> ATAILRPIGLHVEKFQQTYRKKWRFLTSANANVILAEAASGERPARWALTTGMASIPWEYLFFYMSPAEYNRMKNYPGTFAKSASVRIRTWNTRVAFQTGDTQTANATLNQNKFLQVAKGIRSIPFICSTNRKY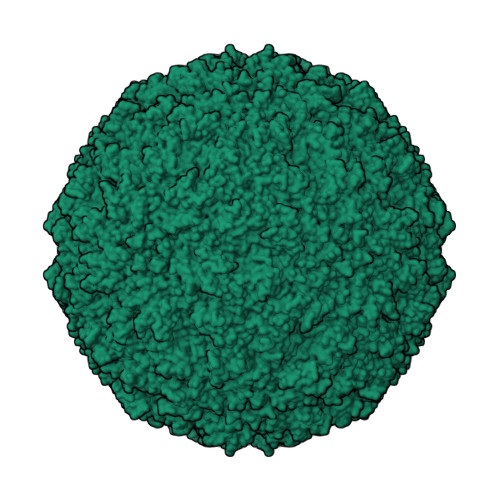TYSDTEPMQPTGFATLTSYEYRDGLKIAMYGYDNDSADFAKKPPADATGAEIYLQDYLTIYTNDARATTGTKILAGFPPYKNFIEEFDASACINTDVVAMDYDFSYAPLVPQFAPVPNNLITQNYNASYPAGTKNEVTAVKTTDSSQATPPTQVRNAPRKYIQGPNADTTFFDEEQNYLRVPIEQGGIFEEVNVETVHDTQMPSINVGIRAVPKLTTIDETTQANSWLDAQGYFEVDCVLTTESVDPYTYIKGGCYSANTKSQLQYFASDGRPIAKVYDNPNVYGRMQMIKTVKP> MVEKEEAGGGISEEEAAQYDRQIRLWGLEAQKRLRASRVLLVGLKGLGAEIAKNLILAGVKGLTMLDHEQVTPEDPGAQFLIRTGSVGRNRAEASLERAQNLNPMVDVKVDTEDIEKKPESFFTQFDAVCLTCCSRDVIVKVDQICHKNSIKFFTGDVFGYHGYTFANLGEHEFVEEKTKVAKVSQGVEDGPDTKRAKLDSSETTMVKKKVVFCPVKEALEVDWSSEKAKAALKRTTSDYFLLQVLLKFRTDKGRDPSSDTYEEDSELLLQIRNDVLDSLGISPDLLPEDFVRYCFSEMAPVCAVVGGILAQEIVKALSQRDPPHNNFFFFDGMKGNGIVECLGPK;> MALSRGLPRELAEAVAGGRVLVVGAGGIGCELLKNLVLTGFSHIDLIDLDTIDVSNLNRQFLFQKKHVGRSKAQVAKESVLQFYPKANIVAYHDSIMNPDYNVEFFRQFILVMNALDNRAARNHVNRMCLAADVPLIESGTAGYLGQVTTIKKGVTECYECHPKPTQRTFPGCTIRNTPSEPIHCIVWAKYLFNQLFGEEDADQEVSPDRADPEAAWEPTEAEARARASNEDGDIKRISTKEWAKSTGYDPVKLFTKLFKDDIRYLLTMDKLWRKRKPPVPLDWAEVQSQGEETNASDQQNEPQLGLKDQQVLDVKSYARLFSKSIETLRVHLAEKGDGAELIWDKDDPSAMDFVTSAANLRMHIFSMNMKSRFDIKSMAGNIIPAIATTNAVIAGLIVLEGLKILSGKIDQCRTIFLNKQPNPRKKLLVPCALDPPNPNCYVCASKPEVTVRLNVHKVTVLTLQDKIVKEKFAMVAPDVQIEDGKGTILISSEEGETEANNHK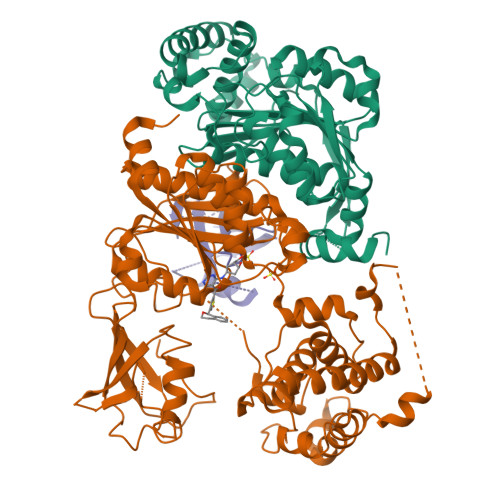KLSEFGIRNGSRLQADDFLQDYTLLINILHSEDLGKDVEFEVVGDAPEKVGPKQAEDAAKSITNGSDDGAQPSTSTAQEQDDVLIVDSDEEDSSNNADVSEEERSRKRKLDEKENLSAKRSRIEQKEELDDVIALD;> MSDQEAKPSTEDLGDKKEGEYIKLKVIGQDSSEIHFKVKMTTHLKKLKESYCQRQGVPMNSLRFLFEGQRIADNHTPKELGMEEEDVIEVYQEQTGGHSTV>[2x]GMGSYQLLVPPPEALSKPLSVPTRLLLGPGPSNLAPRVLAAGSLRMIGHMQKEMLQIM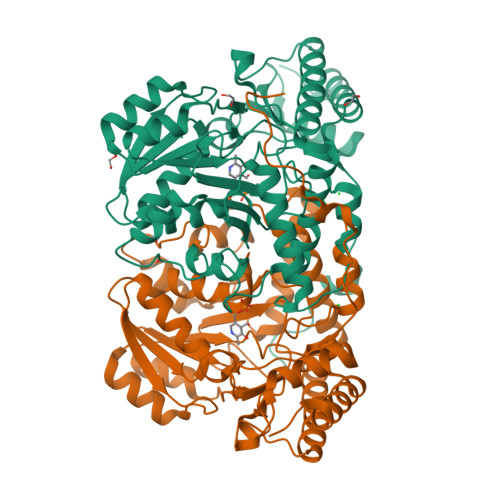EEIKQGIQYVFQTRNPLTLVVSGSGHCAMETALFNLLEPGDSFLTGTNGIWGMRAAEIADRIGARVHQMIKKPGEHYTLQEVEEGLAQHKPVLLFLVHGESSTGVVQPLDGFGELCHRYQCLLLVDSVASLGGVPIYMDQQGIDIMYSSSQKVLNAPPGISLISFNDKAKYKVYSRKTKPVSFYTDITYLAKLWGCEGETRVIHHTTPVTSLYCLRESLALIAEQGLENCWRRHREATAHLHKHLQEMGLKFFVKDPEIRLPTITTVTVPAGYNWRDIVSYVLDHFSIEISGGLGPTEERVLRIGLLGYNATTENVDRVAEALREALQHCPKNKL> MAATVGPESIWLWIGTIGMTLGTLYFVGRGRGVRDRKMQEFYIITTFITTIAAAMYFAMATGFGVTEVVVGDEALTIYWARYADWLFTTPLLLLDLGLLAGANRNTIATLIGLDVFMIGTGMIAAFAATPGTRIAWWGISTGALLALLYVLVGTLSKDARGQSPEVASLFGRLRNLVIVLWLLYPVVWILGTEGTFGILPLYWETAAFM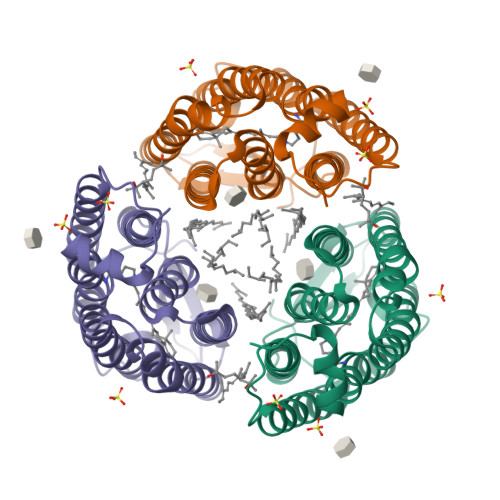VLDLSAKVGFGVVLLRSRSVLRRVVTPTAAPT> MGVNAVHWFRKGLRLHDNPALKECIQGADTIRCVYILDPWFAGSSNVGINRWRFLLQCLEDLDANLRKLNSRLFVIRGQPADVFPRLFKEWNITKLSIEYDSEPFGKERDAAIKKLATEAGVEVIVRISHTLYDLDKIIELNGGQPPLTYKRFQTLVSKMEPLEMPADTITSDVIGKCMTPLSDDHDEKYGVPSLEELGFDTDGLSSAVWPGGETEALTRLERHLERKAWVANFERPRMNANSLLASP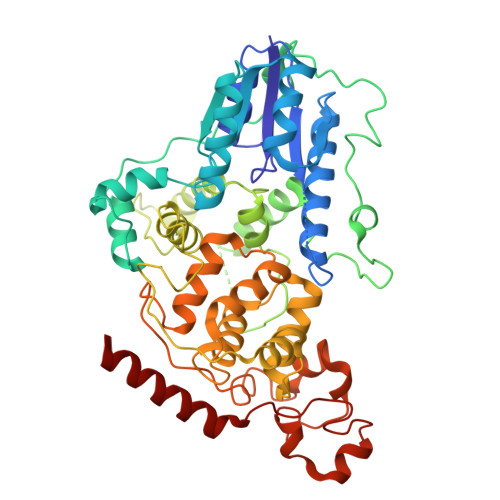TGLSPYLRFGCLSCRLFYFKLTDLYKKVKKNSSPPLSLYGQLLWREFFYTAATNNPRFDKMEGNPICVQIPWDKNPEALAKWAEGRTGFPWIDAIMTQLRQEGWIHHLARHAVACFLTRGDLWISWEEGMKVFEELLLDADWSINAGSWMWLSCSSFFQQFFHCYCPVGFGRRTDPNGDYIRRYLPVLRGFPAKYIYDPWNAPEGIQKVAKCLIGVNYPKPMVNHAEASRLNIERMKQIYQQL>MSEQQVQELEKKWYALQVEPGKENEAKENLLKVLELEGLKDLVDEVIVPAEEKVVIRAQGKEKYRLSLKGNARDISVLGKKGVTTFRIENGEVKVVESVEGDTCVNAPPISKPGQKITCKENKTEAKIVLDNKIFPGYILIKAHMNDK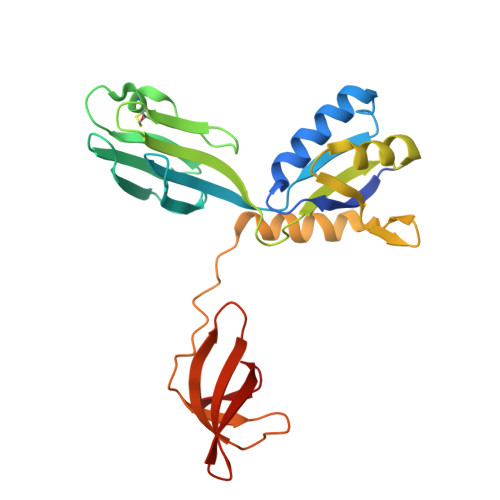LLMAIEKTPHVFRPVMVGGKPVPLKEEEVQNILNQIKRGVKPSKVEFEKGDQVRVIEGPFMNFTGTVEEVHPEKRKLTVMISIFGRMTPVELDFDQVEKI[4x]> AAVRLSVSGTNLNYNGHHIFLSGANQAWVNYARDFGHNQYSKGKSTFESTLSDMQSHGGNSVRVWLHIEGESTPEFDNNGYVTGIDNTLISDMRAYL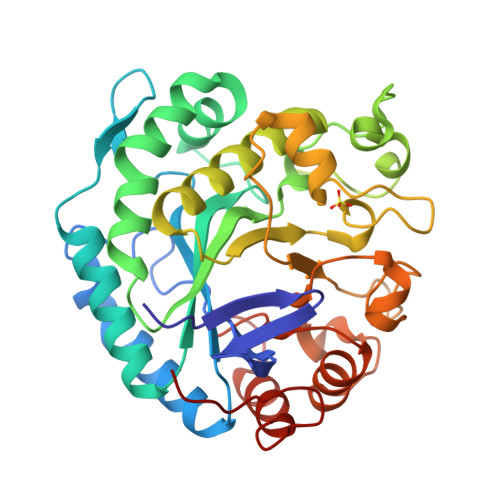HAAQRHNILIFFTLWNGAVKQSTHYRLNGLMVDTRKLQSYIDHALKPMANALKNEKALGGWDIMNEPEGEIKPGESSSEPCFDTRHLSGSGAGWAGHLYSAQEIGRFVNWQAAAIKEVDPGAMVTVGSWNMKADTDAMGFHNLYSDHCLVKAGGKQSGTLSFYQVHTYDWQNHFGNESPFKHSFSNFRLKKPMVIGEFNQEHGAGMSSESMFEWAYTKGYSGAWTWSRTDVSWNNQLRGMQHLKSRTDHGQVQFGL> MAETSNDPFLSYVLSSKQLTNLNRLRRKAVTKQLGSSDDNKVSEEFLRYQHTYQREAFEYLQTKHDAHKIMESQYEQYQ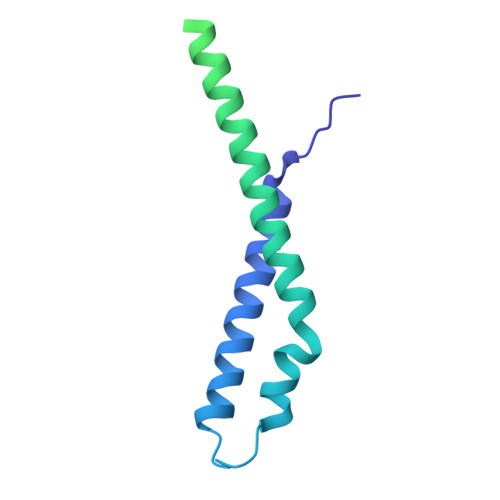SSSKTRRYSIDLDSVDAVDTESQTEYPNEEFIDRNEDSEAVMELRKRLLGKGQNKGLGYETTKSVDRQIEDQDTLQQDLIQDMSKLVGSLKQGAVAFQSALDEDKQVLGAAEIGIQVASQGLMDVSGKLRKYD N-(4-OXO-5,6,7,8-TETRAHYDRO-4H-[1,3]THIAZOLO[5,4-C]AZEPIN-2-YL)ACETAMIDE 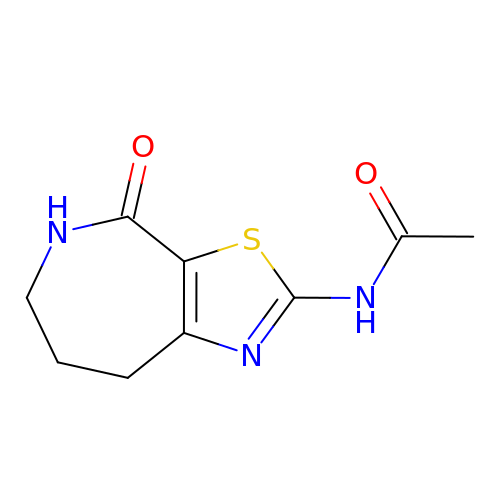| C9 H11 N3 O2 S | OYHOEDBNAJPFKK-UHFFFAOYSA-N> EAPYASLTEIEHLVQSVCKSYRETCQLRLEDLLRQRSNIFSREEVTGYQRKSMWEMWER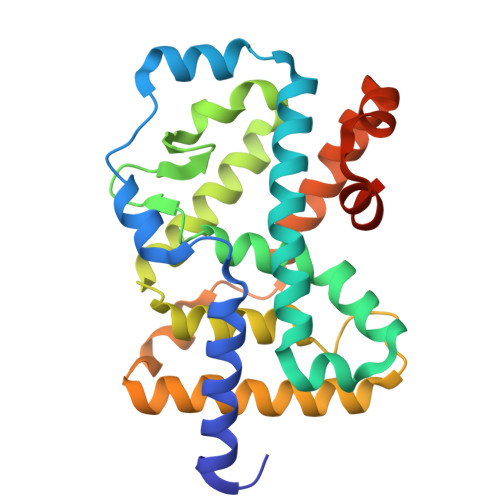CAHHLTEAIQYVVEFAKRLSGFMELCQNDQIVLLKAGAMEVVLVRMCRAYNADNRTVFFEGKYGGMELFRALGCSELISSIFDFSHSLSALHFSEDEIALYTALVLINAHRPGLQEKRKVEQLQYNLELAFHHHLCKTHRQSILAKLPPAGKLASLCSQHVERLQIFQHLHPIVVQAAFPPLYKELFSTETESPVGLSK> MGHHHHHHGSMNPEYDYLFKLLLIGDSGVGKSCLLLRFADDTYTESYISTIGVDFKIRTIELDGKTIKLQIWDTAGQERFRTITS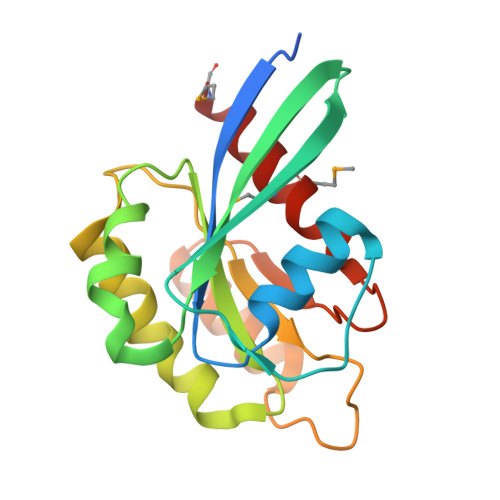SYYRGAHGIIVVYDVTDQESFNNVKQWLQEIDRYASENVNKLLVGNKCDLTTKKVVDYTTAKEFADSLGIPFLETSAKNATNVEQSFMTMAAEIKKRMG> AVANSIVSSVAPGKEPGSLVCIQAKDGKVIGMGARVHCGPATVLVTAGHVLKKGMIADLYLAKYSVSSKEGKRVLMDPTWKIEYGSLNKEADVISVQVPAAVWSRLGVTAARVRKPTVKVPVLAYGGEASGLLQSSQGFATPDGNMSVAHSCSTRPGWSGTPLYAGSDIVAIHRRWEDIGVKNLATNLSIFHANCASSANGEQGAREIDAEEWISREVTPTDVYIAGRGKYRVAGDEFSHSSYDPLAFSKYKKERGEMTWADMVEGDLDWDAREE

Sobemoviruses encode serine-like 3C proteases (Pro) that participate in the processing and maturation of other virus-encoded proteins. Its cis and trans activity is mediated by the naturally unfolded virus-genome-linked protein (VPg). Here, we solved a full Pro–VPg 3D structure of ryegrass mottle virus (RGMoV) that demonstrates the structural changes in three different conformations due to VPg interaction with Pro. The overall fold change of Δ117Pro is typical for CLP and is very similar to the structure of SeMV Pro.

We crystallized and solved 3D crystal structures for two catalytically active forms of Δ117Pro: one in its VPg-free form, the second in its VPg-bound state with fused VPg at the C-terminal part (Δ117Pro-E/A-VPg), and one catalytically defective Δ117Procm form with S159/A mutation. The VPg sequence GEMTWADMVE, corresponding to residues 256–265 in Δ117Pro-E/A-VPg, forms a short α-helix that binds to the surface of Δ117Pro. W260 is a key residue in this interaction; it is located in a very tight and largely hydrophobic pocket, forming a hydrogen bond with the main-chain carbonyl oxygen of D77. The interaction of the VPg helix with Δ117Pro is also ensured by two additional hydrogen bonds: one between the K52 side chain nitrogen and V264 main chain oxygen, and the second between the I82 main chain nitrogen and M258 main chain oxygen. VPg-binding sites are mostly hydrophobic, as they are formed by L51, M55, M76, W80, I82, L87, I94, and V96. The VPg helix is somewhat amphipathic, having W260 and V264 side chains located towards the VPg site, and T259, D262, and E265 side chains exposed to the outside environment, so the VPg–Pro interaction is also strengthened by hydrophobic interactions. The binding of VPg causes several significant conformational shifts in the Δ117Pro structure. However, in the Δ117Pro chain B, Δ117Procm, and Δ117Pro-E/A-VPg cases, D92 is directed towards H49, as would be expected in an active Pro. None of these conformational shifts were observable in SeMV Pro; both the catalytic triad and Glu-binding regions aligned almost perfectly with Δ117Pro-E/A-VPg. Similar major structural changes have not been observed for the closely related SeMV Pro, the in cis active structure, which is very similar to VPg bound, a completely in trans-active RGMoV Pro.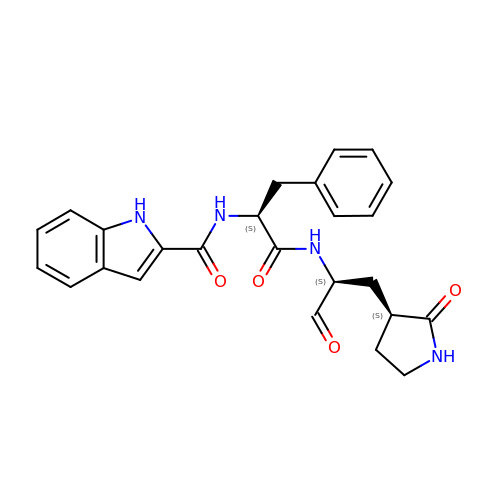~{N}-[(2~{S})-1-oxidanylidene-1-[[(2~{S})-1-oxidanylidene-3-[(3~{S})-2-oxidanylidenepyrrolidin-3-yl]propan-2-yl]amino]-3-phenyl-propan-2-yl]-1~{H}-indole-2-carboxamide | C25 H26 N4 O4 | BRFDPJYHCJVJEP-ZJOUEHCJSA-N>[2x]MKAPVRVAVTGAAGQIGYSLLFRIAAGEMLGKDQPVILQLLEIPQAMKALEGVVMELEDCAFPLLAGLEATDDPKVAFKDADYALLVGAAPRKAGMERRDLLQVNGKIFTEQGRALAE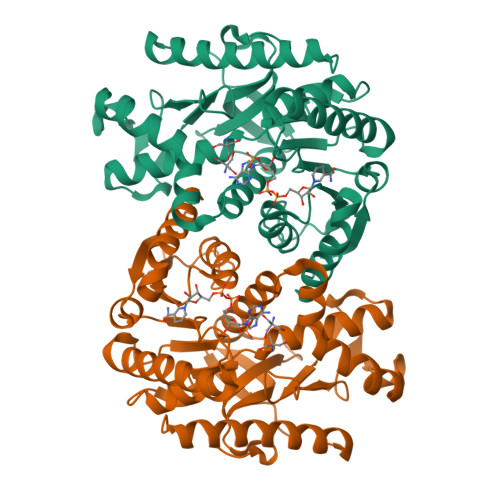VAKKDVKVLVVGNPANTNALIAYKNAPGLNPRNFTAMTRLDHNRAKAQLAKKTGTGVDRIRRMTVWGNHSSTMFPDLFHAEVDGRPALELVDMEWYEKVFIPTVAQRGAAIIQARGASSAASAANAAIEHIRDWALGTPEGDWVSMAVPSQGEYGIPEGIVYSFPVTAKDGAYRVVEGLEINEFARKRMEITAQELLDEMEQVKALGLI>MDKQYPVRQWAHGADLVVSQLEAQGVRQVFGIPGAKIDKVFDSLLDSSIRIIPVRHEANAAFMAAAVGRITGKAGVALVTSGPGCSNLITGMATANSEGDPVVALGGAVKRADKAKQVHQSMDTVAMFSPVTKYAIEVTAPDALAEVVSNAFRAAEQGRPGSAFVSLPQDVVDGPVSGKVLPASGAPQMGAAPDDAIDQVAK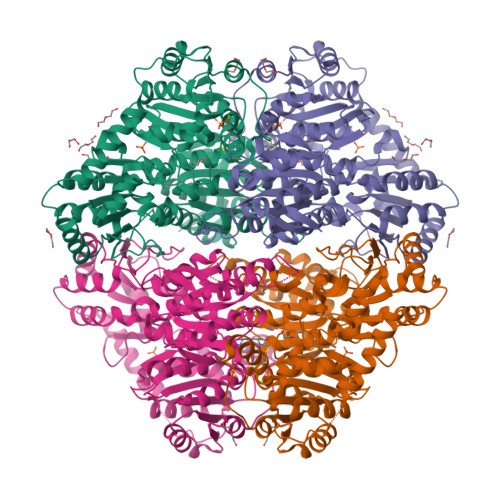LIAQAKNPIFLLGLMASQPENSKALRRLLETSHIPVTSTYQAAGAVNQDNFSRFAGRVGLFNNQAGDRLLQLADLVICIGYSPVEYEPAMWNSGNATLVHIDVLPAYEERNYTPDVELVGDIAGTLNKLAQNIDHRLVLSPQAAEILRDRQHQRELLDRRGAQLNQFALHPLRIVRAMQDIVNSDVTLTVDMGSFHIWIARYLYTFRARQVMISNGQQTMGVALPWAIGAWLVNPERKVVSVSGDGGFLQSSMELETAVRLKANVLHLIWVDNGYNMVAIQEEKKYQRLSGVEFGPMDFKAYAESFGAKGFAVESAEALEPTLRAAMDVDGPAVVAIPVDYRDNPLLMGQLHLSQILEHHHHHH[2x]> ARGTNVGRECCLEYFKGAIPLRKLKTWYQTSEDCSRDAIVFVTVQG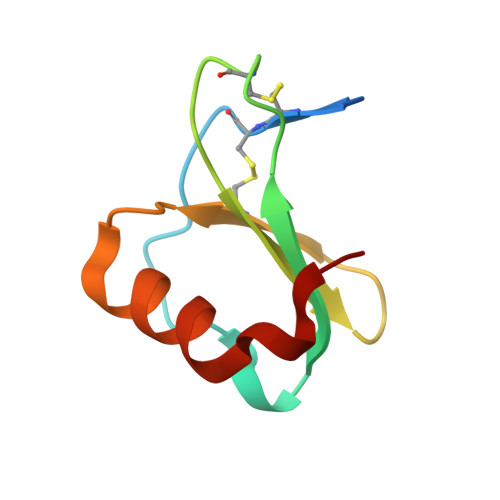RAICSDPNNKRVKNAVKYLQSLERS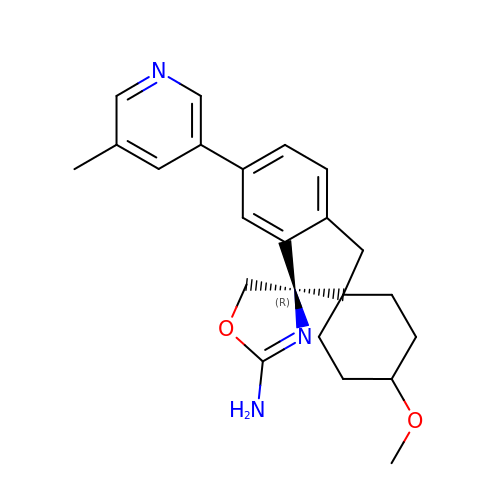(1r,4r)-4-methoxy-6'-(5-methyl-3-pyridinyl)-3'H-dispiro[cyclohexane-1,2'-indene-1',4''-[1,3]oxazol]-2''-amine | C23 H27 N3 O2 | XMEKMASQQBIQCX-VJBMBRPKSA-N>[3x]MTSKREKSLDHTLELKIPFETERQAT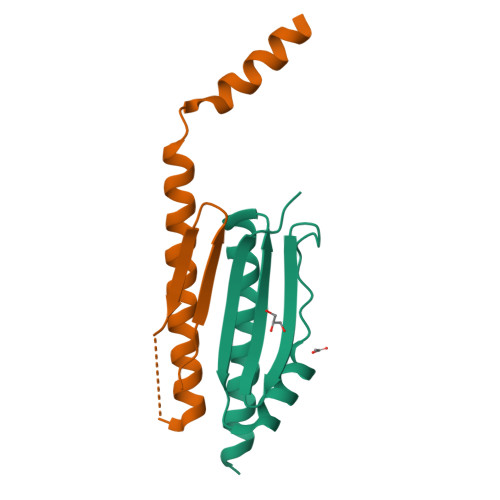IATKVLSPDPILKPQDFQVDYSSEKNVMLVQFRSIDDRVLRVGVSSIIDSIKTIVEAMDVLSHHHHHH;>[3x]MKLPVAQYSAPDGVEKSFAPIRDDPRYMTTEGRTTGPSDHVLNAGQIDRDKPSEPERTKDGSQLTYLGQLRTQLTGLQDDINEFLTGRMELAKNKKKAGADEKRIQEEINQLLDGGDGDEDAV> MFKNALRRAGVAAPRISRVAQRGYAEAKATPTEVTSILEERIRGVSGEAN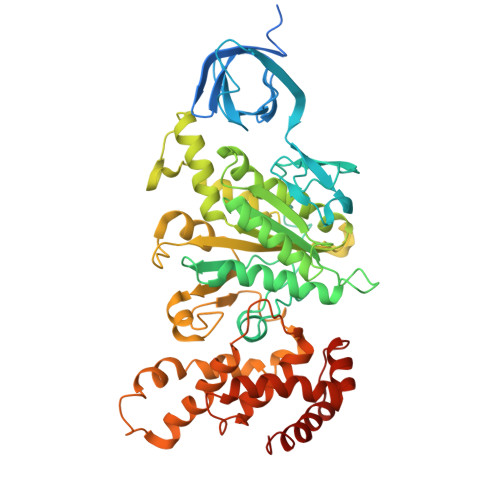LNETGRVLSVGDGIARVFGLNNIQAEELVEFASGVKGMALNLEAGQVGIVLFGSDRLVKEGETVKRSGSIVDVPVGPALLGRVVDALGNPIDGKGPIETEFRIRAQVKAPGILPRTSVNEPMQTGLKAVDALVPIGRGQRELIIGDRQTGKTQIAIDTILNQKRWNYGQDEKKKLYCVYVAVGQKRSTVAQLVQTLEHHDALKYSIIVAATASEAAPLQYLAPFTGTAMGEWFRDNGKGALIVFDDLSKQAVAYRQMSLLLRRPPGREAYPGDVFYLHSRLLERAAKMNEREGGGSLTALPIIETQGGDVSAYIPTNVISITDGQIFLEAELFYKGIRPAINVGLSVSRVGSAAQVKAMKQVAGSLKLFLAQYREVAAFAQFGSDLDASTKQTLTRGERLTLLLKQKQASPMSSEEMVPLIYAGVNGYIDNIPVKQVEKFEAEFVSYLHANESDLLKDIAATGELSKENLEKLKSITENFVGSFAK> GSHMTKYKYTVEESERFNKHGIDLTVYGQVDPSATVVRVSVERGHFQEFFNVRSSYTYYVVSGQGVFYLNSEAVPAGATDLITVPPNTRIHYFGSMEMVLTVAPAFNEQDERH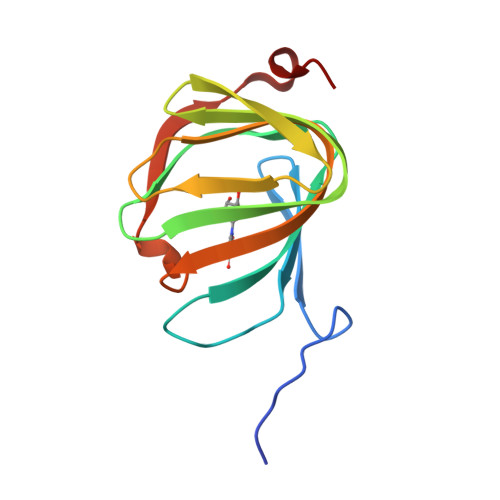VRFISESESPY(2~{S})-~{N}-[[4-(aminomethyl)phenyl]methyl]-1-[(2~{R})-2-azanyl-3-phenyl-propanoyl]pyrrolidine-2-carboxamide 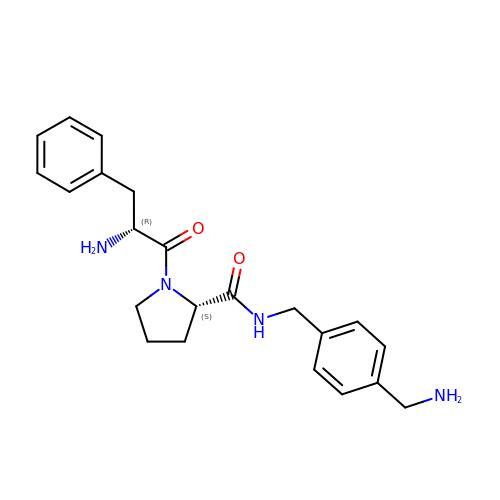| C22 H28 N4 O2 | MTUGEKUGFKKRIV-UXHICEINSA-N>[2x]MQNAEKLDFKITGGWIIDGTGAPRRRADLGVRDGRIAAIGELGAHPARHAWDASGKIVAPGFIDVHGHDDLMFVEKPDLRWKTSQGITTVVVGNCGVSAAPAPLPGNTAAALALLGETPLFADVPAYFAALDAQRPMINV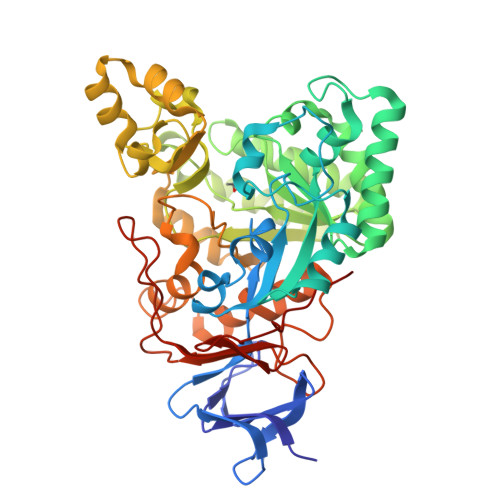AALVGHANLRLAAMRDPQAAPTAAEQQAMQDMLQAALEAGAVGFSTGLAYQPGAVAQAAELEGLARVAAERRRLHTSHIRNEADGVEAAVEEVLAIGRGTGCATVVSHHKCMMPQNWGRSRATLANIDRAREQGVEVALDIYPYPGSSTILIPERAETIDDIRITWSTPHPECSGEYLADIAARWGCDKTTAARRLAPAGAIYFAMDEDEVKRIFQHPCCMVGSDGLPNDARPHPRLWGSFTRVLGRYVREARLMTLEQAVARMTALPARVFGFAERGVLQPGAWADVVVFDPDTVADRATWDEPTLASVGIAGVLVNGAEVFPQPPADGRPGQVLRAGA> MDIGIDSDPQKTNAVPRPKLVVGLVVDQMRWDYLYRYYSKYGEGGFKRMLNTGYSLNNVHIDYVPTVSAIGHTSIFTGSVPSIHGIAGADWYDKELGKSVYCTSDETVQPVGTTSNSVGQHSPRNLWSTTVTDQLGLATNFTSKVVGVSLADAASILPAGHNPTGAFWFDDTTGKFITSTYYTKELPKWVN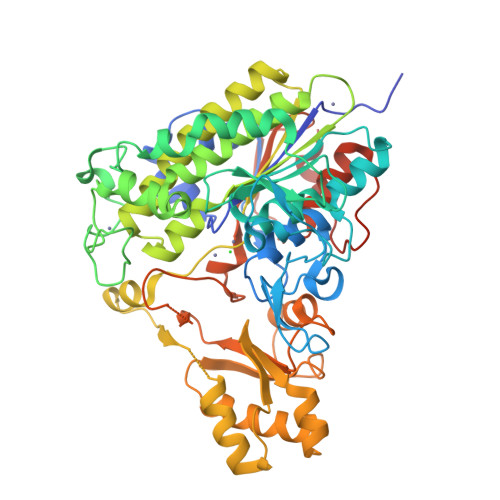DFNNKNVPAQLVANGWNTLLPINQYTESSEDNVEWEGLLGSKKTPTFPYTDLAKDYEAKKGLIRTTPFGNTLTLQMADAAIDGNQMGVDDITDFLTVNLASTDYVGHNFGPNSIEVEDTYLRLDRDLADFFNNLDKKVGKGNYLVFLSADHGAAHSVGFMQAHKMPTGFFVEDMKKEMNAKLKQKFGADNIIAAAMNYQVYFDRKVLADSKLELDDVRDYVMTELKKEPSVLYVLSTDEIWESSIPEPIKSRVINGYNWKRSGDIQIISKDGYLSAYSKKGTTHSVWNSYDSHIPLLFMGWGIKQGESNQPYHMTDIAPTVSSLLKIQFPSGAVGKPITEVIGRIEGRSAWSHPQFEK>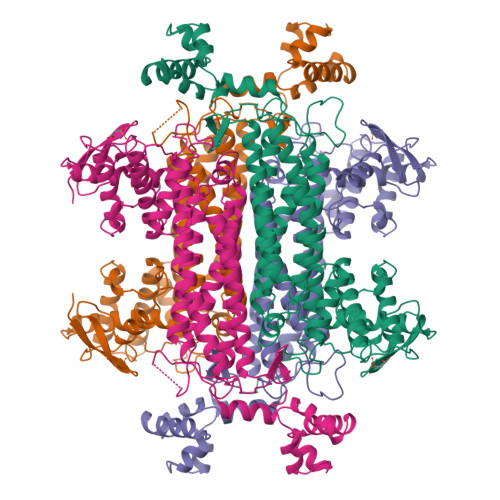[2x]MNTVRSEKDSMGAIDVPADKLWGAQTQRSLEHFRISTEKMPTSLIHALALTKRAAAKVNEDLGLLSEEKASAIRQAADEVLAGQHDDEFPLAIWQTGSGTQSNMNMNEVLANRASELLGGVRGMERKVHPNDDVNKSQSSNDVFPTAMHVAALLALRKQLIPQLKTLTQTLNEKSRAFADIVKIGRTNLQDATPLTLGQEISGWVAMLEHNLKHIEYSLPHVAELALGGTAVGTGLNTHPEYARRVADELAVITCAPFVTAPNKFEALATCDALVQAHGALKGLAASLMKIANDVRWLASGPRCGIGEISIPENEPGSSIMPGKVNPTQCEALTMLCCQVMGNDVAINMGGASGNFELNVFRPMVIHNFLQSVRLLADGMESFNKHCAVGIEPNRERINQLLNESLMLVTALNTHIGYDKAAEIAKKAHKEGLTLKAAALALGYLSEAEFDSWVRPEQMVGSMKAGR>[2x]MGEKITEEREFQSISEIPEEEIDATNDEEKLADIVENEIEKEIRKSKTRKCKTIENFYYYILRDGKIYPASDYDIEVEKGKRSANDIYAFVETDVTRDFDEFLFDIDYGLPSISDILKFYLEKAGFRIANEVPTPNLKYYIHAVVEFGEDRPQYLAVNIYDIDSLARALRIPQIVEQKLGNKPRTITADEFNDIERIVAEEQPILAGYTYDEALRIPYHYYVDHNNSFKDDALKIAHAYLQLFPTPYQVCYEWKARWFNKIDCLKLERLKPSSHHHHHH

Acidianus two-tailed virus (ATV) infects crenarchaea of the genus Acidianus living in terrestrial thermal springs at extremely high temperatures and low pH. ATV is a member of the Bicaudaviridae virus family and undergoes extra-cellular development of two tails, a process that is unique in the viral world. ATV is the fourth most abundant of these proteins. Remarkably, ATV displays a new protein fold, consistent with the absence of homologues of this protein in public sequence databases.

The crystals of the second form reached a 2.15 Å diffraction limit and comprised two monomers in its asymmetric unit. The current model is refined against native data to 2.15 Å, resulting in an R/R factors of 20.2%/23.4% and includes residues 22 to 270 in monomer A and 25 to 269 in monomer B. Two loops could not be built in the model owing to the lack of supporting electron density. The first of these loops comprises residues Ser46 to Thr53 in monomer A and Arg44 to Ile54 in monomer B, whereas the second missing loop encompases residues Gly148 to Arg151 in both monomers. The structure of an ATV monomer is made up of 10 helices and two -sheets, one composed of seven strands and the other consisting of two short parallel strands. As expected for a hyperthermostable protein, the ATV monomer is stabilised by a relatively high number of salt bridges (5 in monomer A and 8 in monomer B; to be considered as engaged in a salt bridge, the centroids of the side-chain charged groups and at least a pair of side-chain nitrogen and oxygen atoms of the ion-pairing residues must be within a 4 Å distance). Some of these salt bridges form networks, namely the triplets Glu29/Asp33/Lys260 and Glu252/Lys254/Lys265 in monomer B, another feature related to hyperthermostability. Furthermore, a disulphide bond is observed between cysteines 250 and 263 in both monomers. The analysis of the crystal interfaces present in the second crystal form with the PISA software suggested two possible dimers with a significant buried area at the interface, namely 1258 Å2 and 1087 Å2 per monomer, respectively. In the closed dimer the concave sides of the monomers face each other thereby creating a chamber with a volume of 8650 Å3. Finally, the two interfaces identified in the second-form crystals of ATV are assembled head-to-tail, resulting in helicoidal fibers that extend indefinitely along the crystallographic c-axis.>ALVFFAEDAAIIGLMV[16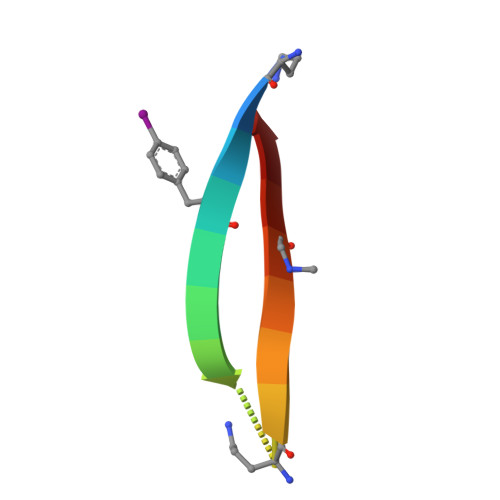x]(2R,3S,4s,5R,6S)-2,3,4,5,6-pentahydroxycyclohexanone 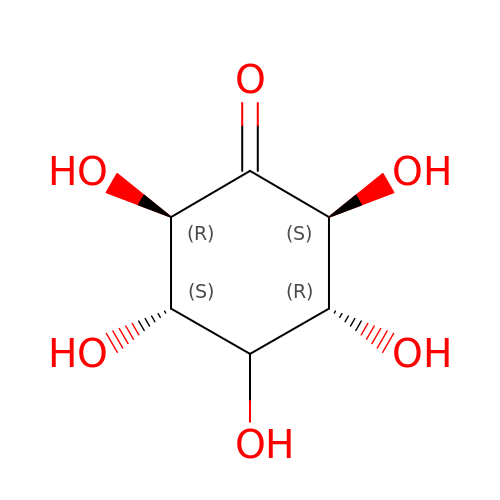| C6 H10 O6 | VYEGBDHSGHXOGT-HYFGLKJPSA-N> PPALHLVDPQIQLTITDPKVYPIILRLGSNLSLSMARRNLDSLEARAFQSTPIVVQ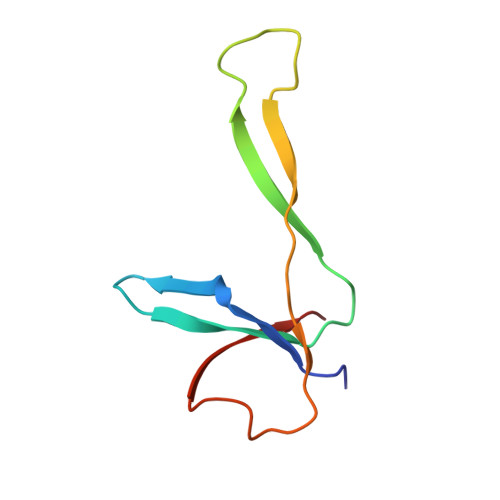MTKLATTEELPDEFVVVTAK> ADLPGKGITVNPVQSTITEETFQTLLVSRALEKLGYTVNKPSEVDYNVGYTSLASGDATFTAVNWTPLHDNMYEAAGGDKKFYREGVFVNGAAQGYLIDKKTADQYKITNIAQLKDPKIAKLFDTNGDGKADLTGCNPGWGCEGAINHQLAAYELTNTVTHNQGNYAAMMADTISRYKEGKPVFYYTWTPYWVSNELKPGKDVVWLQVPFSALPGDKNADTKLPNGANYGFPVSTMHIVANKAWAEKNPAAAKLFAIMQLPVADI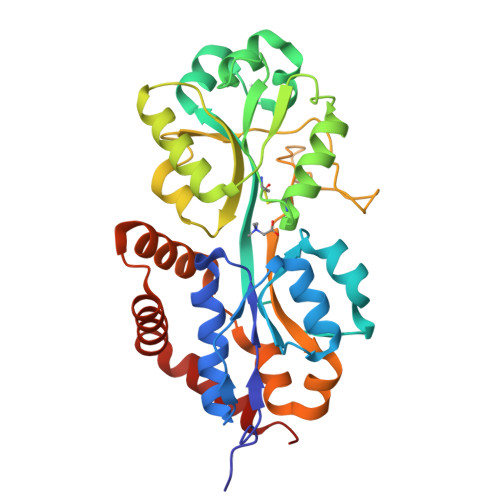NAQNAIMHDGKASEGDIQGHVDGWIKAHQQQFDGWVNEALAAQK> MRDPFMEALGLKVLHLAPGEAVVAGEVRADHLNLHGTAHGGFLYALADSAFALASNTRGPAVALSCRMDYFRPLGAGA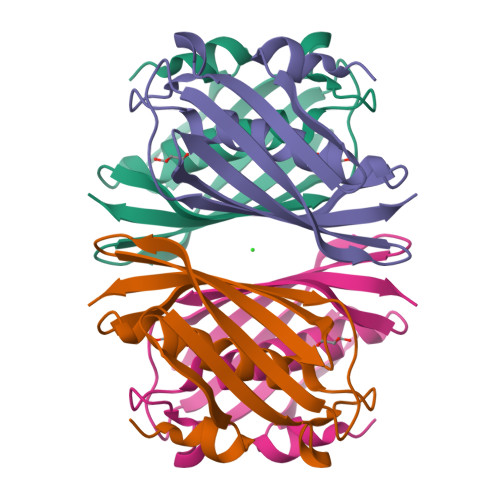RVEARAVEVNLSRRTATYRVEVVSEGKLVALFTGTVFRLGGDGDDVPAGTGNLAPREA> TMAKVLAVDDSISIRQMVSHTLQDAGYEVETAADGREALAKAQKARFDVIISDVNMPVMTGFEFVKAVRMQSQYKFTPILMLTTETSPEKKQEGKAV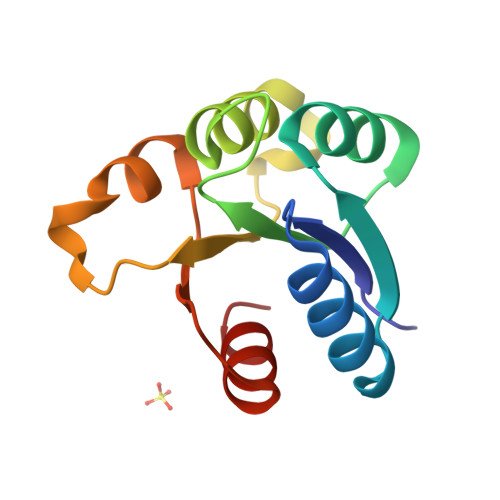GATGWLVKPFNPETLLKTLQRVL> GAMGQDWRADYHSRIGEQRRLTLADGTQVQLNTDSALNVAFDQQARRLRLVRGEMLITRPALADSRPLWVDTEHGRLESTLAQFNVRLHGQHTQATVYQGSVALQPALHAYPPILLGA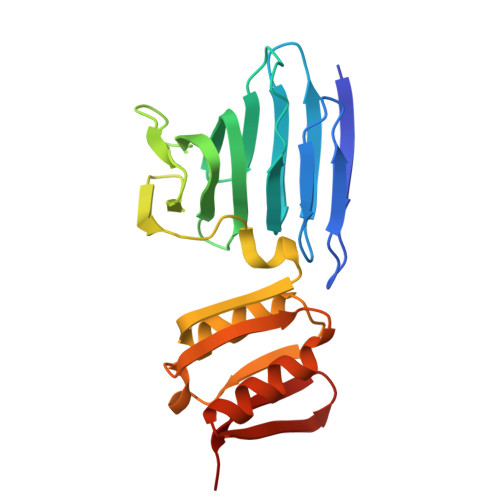GEQASFNQQGLLARQAVAAVAPAWSQGMLVAQGQPLAAFIEDLARYRRGHLACDPALAGLRVSGTFPLENTDKIIAAVAETLQLEVQHFTRYWVTLKPRMA>[2x]MGDT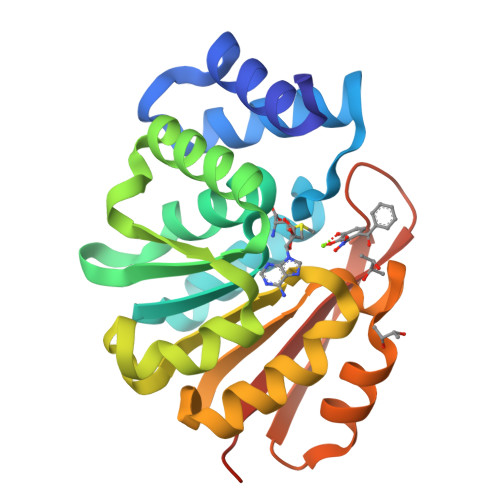KEQRILRYVQQNAKPGDPQSVLEAIDTYCTQKEWAMNVGDAKGQIMDAVIREYSPSLVLELGAYCGYSAVRMARLLQPGARLLTMEMNPDYAAITQQMLNFAGLQDKVTILNGASQDLIPQLKKKYDVDTLDMVFLDHWKDRYLPDTLLLEKCGLLRKGTVLLADNVIVPGTPDFLAYVRGSSSFECTHYSSYLEYMKVVDGLEKAIYQGPSSPDKS> SIPVRGAAIFNENLSKILLVQGTESDSWSFPRGKISKDEN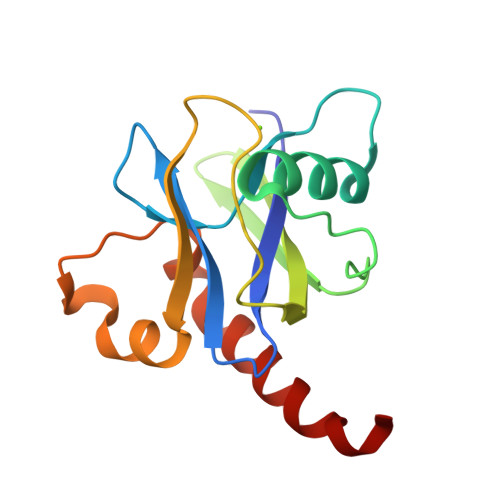DIDCCIREVKEEIGFDLTDYIDDNQFIERNIQGKNYKIFLISGVSEVFNFKPQVRNEIDKIEWFDFKKISKTMYKSNIKYYLINSMMRPLSMWLRHQRQIKNED SLC26A2 is a vital solute carrier responsible for transporting essential nutritional ions, including sulfate, within the human body. SLC26A2 is known to function as an electroneutral anion exchanger, facilitating the exchange of various substrates such as SO42− and C2O42− for Cl−, hydroxide (OH−), or even with each other. Like its homologs, SLC26A2 forms a domain-swapped homodimer. Each protomer of SLC26A2 can be divided into three regions: the N-terminal region (residues 1–104) comprising a few flexible cytosolic helices and loops, the transmembrane domain (TMD, residues 105–540) with 14 transmembrane helices (TMs), and the C-terminal cytosolic sulfate transporter and anti-sigma factor antagonist domain (STAS, residues 541–739).

We purified the overexpressed SLC26A2 in Lauryl Maltose Neopentyl Glycol (LMNG) detergent with 150 mM NaCl at pH 7.5 and then determined the structure, termed SLC26A2-Cl-, by cryo-EM. The final reconstruction achieved a resolution of ~3.2 Å, with sufficient quality for model building. The resulting model covers residues 52–724 without several flexible loops containing residues 186–210, 319–333, and 617–644. We found that the vertical position of TM3/TM10 in SLC26A2 closely resembles that of inward-facing SLC26A9. The result shows that our SLC26A2 structure is open to the cytosolic side and closed to the extracellular side. Notably, in the structure of SLC26A2-Cl-, we identified a distinct density corresponding to the Cl- ion in this cleft. Interestingly, this Cl- does not interact strongly with any surrounding residues. Within 5 Å distance from the Cl-, there are five hydrophobic residues: Y129 from TM1, V167, G166, F165 from the end of TM3, and L491 from TM12. The primary binding force for Cl- appears to be the weak TM3 and TM10 helical dipoles with positive charges pointing towards the substrate-binding pocket. When such distance is between 3.5 and 8 Å, the Cl- ion is within the TM3/TM10 cleft and considered bound. Combining data from three individual runs, we estimated that the substrate-binding pocket is occupied by Cl- ~82 ± 4% of the time.

>[2x]HRILIERQEKSDTNFKEFVIKKLQKNCQCSPAKAKNMILGFLPVLQWLPKYDLKKNILGDVMSGLIVGILLVPQSIAYSLLAGQEPVYGLYTSFFASIIYFLLGTSRHISVGIFGVLCLMIGETVDRELQKAGYDNAHSAPSLGMVSNGSTLLNHTSDRICDKSCYAIMVGSTVTFIAGVYQVAMGFFQVGFVSVYLSDALLSGFVTGASFTILTSQAKYLLGLNLPRTNGVGSLITTWIHVFRNIHKTNLCDLITSLLCLLVLLPTKELNEHFKSKLKAPIPIELVVVVAATLASHFGKLHENYNSSIAGHIPTGFMPPKVPEWNLIPSVAVDAIAISIIGFAITVSLSEMFAKKHGYTVKANQEMYAIGFCNIIPSFFHCFTTSAALAKTLVKESTGCHTQLSGVVTALVLLLVLLVIAPLFYSLQKSVLGVITIVNLRGALRKFRDLPKMWSISRMDTVIWFVTMLSSALLSTEIGLLVGVCFSIFCVILRTQKPKSSLLGLVEESEVFESVSAYKNLQIKPGIKIFRFVAPLYYINKECFKSALYKQTVNPILIKVAWKKAAKRKIKEKVVTLGGIQDEMSVQLSHDPLELHTIVIDCSAIQFLDTAGIHTLKEVRRDYEAIGIQVLLAQCNPTVRDSLTNGEYCKKEEENLLFYSVYEAMAFAEVSKN Modification dependent restriction endonucleases (MDREs) specifically target DNA that is modified, and are non-toxic to a host with non-modified DNA. Many modification-dependent restriction endonucleases (MDREs) are fusions of a PUA superfamily modification sensor domain and a nuclease catalytic domain. EVE domains belong to the PUA superfamily, and are present in MDREs in combination with HNH nuclease domains. In all crystal structures, VcaM4I protomers have the predicted two domain architecture, with N-terminal domains of the PUA superfamily (residues 1–147), linker helices (148–178), and C-terminal HNH domains (residues 179–309).

The crystal structures of VcaM4I in complex with single- and double-stranded DNA presented here indicate that the domains may also be used for binding of modified DNA. Single-stranded DNAs are bound very similarly to the proximal strand of dsDNA. The ssDNA and dsDNA molecules in the crystals are bound to the N-terminal domains. The other structures were solved by molecular replacement. Except for the weaker diffracting crystals of VcaM4I with dsDNA, the resolution of the data reached around 1.5 Å. Although crystals without DNA, with ssDNA, and with dsDNA grew in different space groups, the protein conformation was remarkably similar in all structures, with the exception of two loops in proximity of the DNA (residues 24–34 and 72–84). The DNA binding site of the C-terminal HNH domains is consistently empty in all structures.

> MNYWWVSQKQTFKQEFEGGYMWSPKENKNGTQSHYYNNMTLVQPGDVVFSFANGLILSVGIARSHAYSYNKPTEFGVAGADWANDGWKIDLEYHLVENKIRPKAHIDFIRPYLPQKYSPLQDNGNGNQAYLFSVPHELASKVVELIGSEAEEVIFGFADTTEITTTADAIECQISNDASIDETEKHQLVKSRRGQGIFRSRLEQVESRCRVTGVQLKNHLIASHIKPWAVSNNQERLDGHNGLLLAPHVDHLFDKGFISFEDNGEMIVSEKLNLDVLKAWSISQGNYGYFSKQQQEYMCYHRENVFKKL> SHRNEAGHGDLHEILHEAVPLDANEREILELKED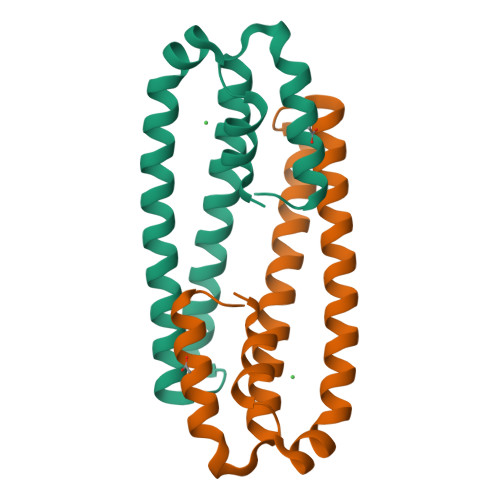AFAQRRREIETRLRAANGKLADAIAKNPAWSPEVEAATQEVERAAGDLQRATLVHVFEMRAGLKPEHRPAYDRVLIDALRRGSQ>[2x]HHHHHHMPRSVTADASGSFLTLTFEDGSESRFHAIWLRDNALDPETRSPGNGQRLITIGDIPADTRISTALVDDGALTVTFAPEGKTVTFPGKWLKSNAYDTDQSSEVGRTSPDVETWDSSQPAPAFDWNEVQSDPKAKRDWLDAIARLGFAKLVNGPVREGALIECASMFGFVRETNYGKYFEVRTEVNPTNLAYTGLGLQAHTDNPYRDPVPSLQILYCLENSAEG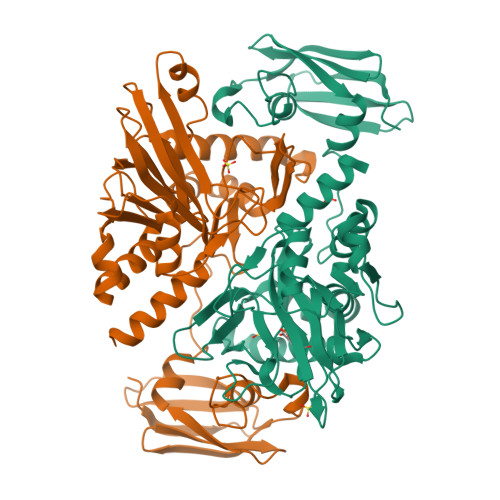GDSIVVDGFRAAERLRDEDPEGFALLAGNPARFEYKGSDGVHLRARRPMIELSPDGEMIAIRFNNRSSAPFVDIPFEKMEAYYAAYRRLGEFIDDPEMGVSFKLEPGESFIVDNTRVLHARLGYSGSGSRWLQGCYADKDGLFSTLNVLNAQLGG>MESLSEVSVQFSQ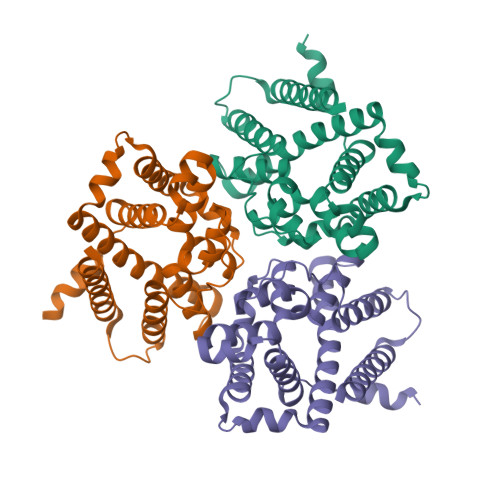LSMFPFFDMAHYLASVMSAREQAGALDIASHSPMASWFSAMLHCFGGGILSSILLAEPPVGILANTTNIMLASAIWYMVYYFPYDLFYNCFFFLPIRLIAAGMKEVTRTWKILSGITHAHSHYKDAWLVMITIGWARGAGGGLISNFEQLVRGVWKPESNEFLKMSYPVKVTLIGAVLFTLQHGHYLPISRHNLMFIYTMFLVSIKVTMMLTHSAGSPFLPLETPLHRILFGLRQNQAEVRESPSSSGAKGKPSKKTLDKDSGEQSNKKDKAAAENLYFQGLEDYKDDDDKHHHHHHHHHH[12x]>[2x]MGSDKIHHHHHHMADTAPQLKRKREQEAEEAETPSTEEKEAGVGNGTSAPVRLPFSGFRVQKVLRESARDKIIFLHGKVNEDSGDTHGEDAVVILEKTPFQVEHVAQLLTGSPELKLQFSNDIYSTYNLFPPRHLSDIKTTVVYPATEKHLQKYMRQDLRLIRETGDDYRTITLPYLESQSLSIQWVYNILDKKAEADRIVFENPDPSDGFVLIPDLKWNQQ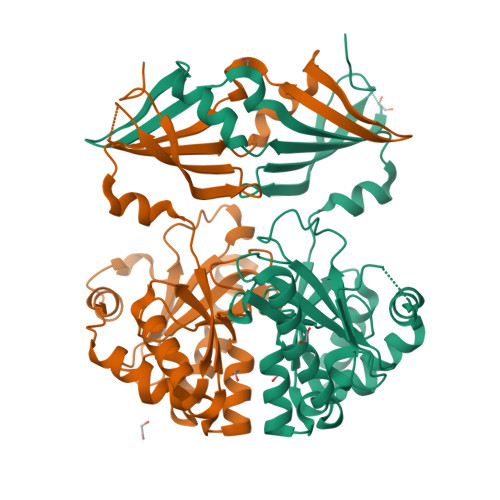QLDDLYLIAICHRRGIRSLRDLTPEHLPLLRNILREGQEAILKRYQVTGDRLRVYLHYLPSYYHLHVHFTALGFEAPGSGVERAHLLAQVIENLECDPKHYQQRTLTFALRTDDPLLQLLQKAQQERN2-hydroxy-1-(4-(isoquinolin-5-yl)piperazin-1-yl)-2-methyl-3-(3-methyl-4-phenyl-1H-pyrazol-1-yl)propan-1-one 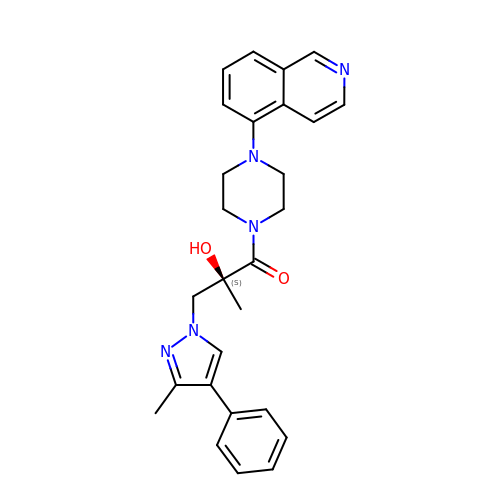| C27 H29 N5 O2 | NIAOQHXCKBVCFC-MHZLTWQESA-N> GAMDPEFSAQLGAMQHLKDQLEQRTRMIEANIHRQ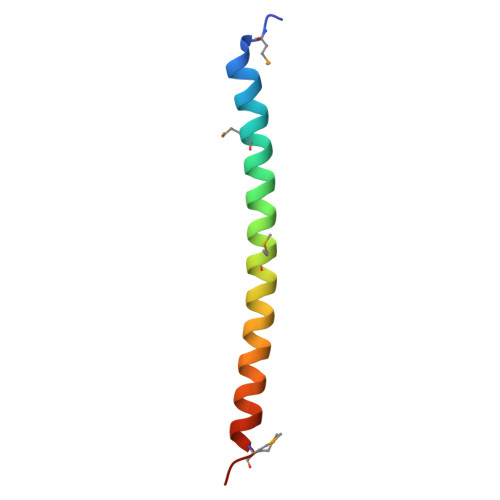QEELRKIQEQLQMVHG>GAMGSKPDTHRADERRFLDERGSSGPLAPNGLNPATIMEKAVRERIVESYF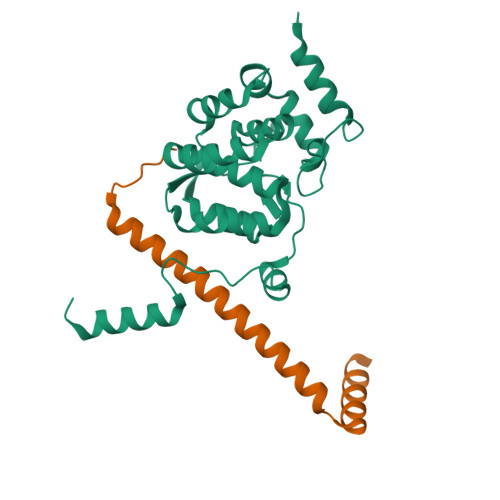WKEQCFGVNEADIVDRVVEHVRFVGGVTGVTQKPSPFLCLAFKLLQLAPGDDILKEYLYFGGEKFKYLRALAAFYIRLTRPDKEVYTLLEPFLEDRRKLRRKGKNGTSLTYMDEFIDDLLTKDRVCSTSLWKMRRRDILEDLDLLEPRVSPLGSLEDILEEEEQAAKNEDGE[2x];>[2x]GAMGTTDDVDPEAEYAAWKLRELRRLRRERDAIEARERELAELERRRNLTEEERRAEDEAHLAKQKAEKESRGKMGYLQKYFHR> MAKRKIQRYVRKDGKCNVHHGNVRETYRYLTDIFTTLVDLKWRFNLLIFVMVYTVTWLFFGMIWWLIAYIRGDMDHIEDPSWTPCVTNLNGFVSAFLFSIETETTIGYGYRVITDKCPEGIILLLIQSVLGSIVNAFMVGCMFVKISQPKKRAETLVFSTHAVISMRDGKLCLMFRVGNLRNSHIVEASIRAKLIKSKQTSEGEFIPLNQTDINVGYYTGDDRLFLVSPLIISHEINQQSPFWEISKAQLPKEELEIVVILEGM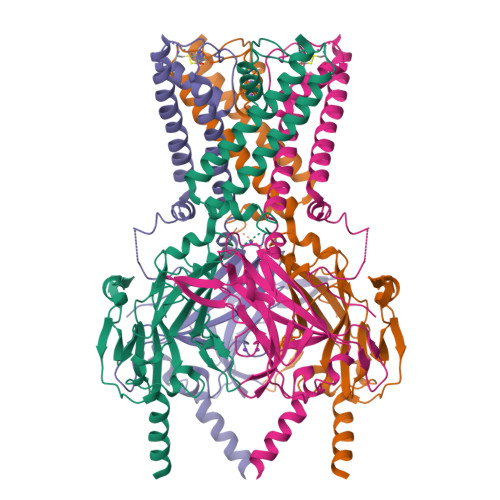VEATGMTCQARSSYITSEILWGYRFTPVLTLEDGFYEVDYNSFHETYETSTPSLSAKELAELANRAESNSLEVLFQ>[14x]AEPVYPDQLRLFSLGQGVCGDKYRPVNREEAQSVKSNIVGMMGQWQISGLANGWVIMGPGYNGEIKPGTASNTWCYPTNPVTGEIPTLSALDIPDGDEVDVQWRLVHDSANFIKPTSYLAHYLGYAWVGGNHSQYVGEDMDVTRDGDGWVIRGNNDGGCDGYRCGDKTAIKVSNFAYNLDPDSFKHGDVTQSDRQLVKTVVGWAVNDSDTPQSGYDVTLRGDTATNWSKTNTYGLSEKVTTKNKFKWPLVGETELSIEIAANQSWASQNGGSTTTSLSQSVRPTVPARSKIPVKIELYKADISYPYEFKADVSYDLTLSGFLRWGGNAWYTHPDNRPNWNHTFVIGPYKDKASSIRYQWDKRYIPGEVKWWDWNWTIQQNGLSTMQNNLARVLRPVRAGITGDFSAESQFAGNIEIGAPVPLAADSKVRRARSVDGAGQGLRLEIPLDAQELSGLGFNNVSLSVTPAANQLEHHHHHH

Aerolysin is a β-pore-forming toxin produced by most Aeromonas bacteria, which has attracted large attention in the field of nanopore sensing due to its narrow and charged pore lumen. Pore-forming toxins (PFTs) are important virulence factors of many pathogenic bacteria, which are secreted in a soluble form and upon host membrane binding, they oligomerize into transmembrane pores undergoing a complex structural reorganization. Domains 3 and 4 form the 120 Å long 14-stranded β-barrel, with each protomer contributing two antiparallel β-strands. Four distinct constriction rings, two at each end of the pore, were identified from the structures and confirmed by MD simulation.

Here, we present the first high-resolution cryo-EM maps and atomic models of WT aerolysin in a membrane-like environment and its Y221G prepore-like mutant. Upon prepore assembly, domains 1 and 2 of adjacent protomers interact through a series of salt bridges and H-bonds that greatly stabilize the cap region. Furthermore, the formation of the concentric β-barrel fold contributes to the stabilization of the prepore through the addition of over 10 H-bonds per subunit. Interestingly, five H-bonds consolidate the lumen of the concentric β-barrel being present both in the prepore and pore configuration. The prepore stability is further enhanced by the hydrophobic residues at the interface of the two β-barrels. Pore formation retains the tight network of bonds between protomers observed in the prepore, while introducing several additional interactions at the folded hinge regions. Overall, previously unseen interactions between side chain and backbone atoms can be observed in both prepore and pore conformations of aerolysin structures at high resolution.> DVSFRLSGADPRSYGMFIKDLRNALPFREKVYNIPLLLPS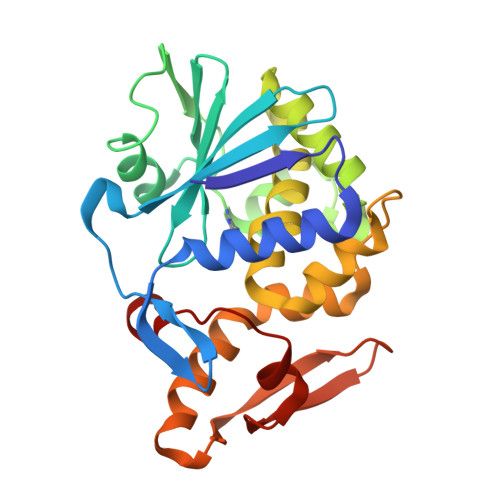VSGAGRYLLMHLFNYDGKTITVAVDVTNVYIMGYLADTTSYFFNEPAAELASQYVFRDARRKITLPYSGNYERLQIAAGKPREKIPIGLPALDSAISTLLHYDSTAAAGALLVLIQTTAEAARFKYIEQQIQERAYRDEVPSLATISLENSWSGLSKQIQLAQGNNGIFRTPIVLVDNKGNRVQITNVTSKVVTSNIQLLLNTRNI>GPSGGGADVNKGPWAMALTPMEFARKYNLLRKDDALLDNPVPGEEMTAGIRRGDAKRVFTMQLGPYWDGFEECSPQAYALSAVFMARMNRDRDAANNILKVLDKTFVDGKPDFSVARPVMKKYQNSELVQEVVAKHAYVLTVIASLLEAAREDGVVPSSEFLWLKPVDRRLWYMLNCVGRQTPYSEVAGPFAHWKAE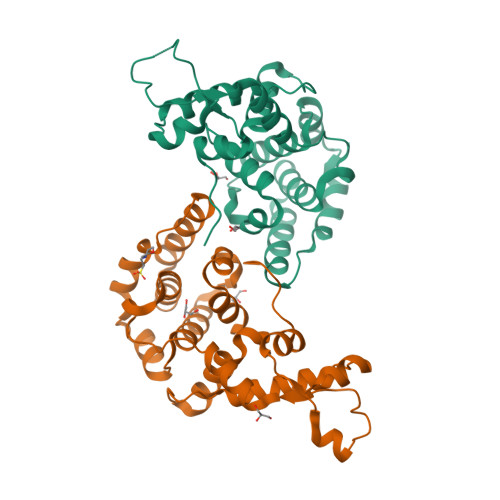KEMGRRSLVPMIDEAIRALEIAVKEVRLTPRQMEELEP[2x]> SACKFEEGQDVLARWSDGLFYLGTIKKINILKQSCFIIFEDSSKSWVLWKDIQTGATGSGEMVCTICQEEYSEAPNEMVICDKCGQGYHQLCHTPHIDCSVIDSDEKWLCRQCVFATTTKRGGALKKGPNAKALQVMKQTLPYSV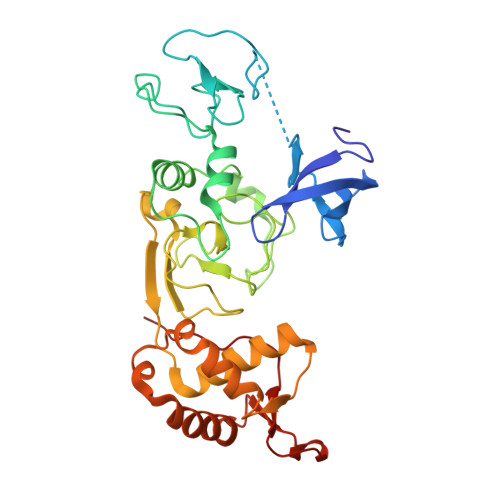ADLEWDAGHKTNVQQCYCYCGGPGDWYLKMLQCCKCKQWFHEACVQCLQKPMLFGDRFYTFICSVCSSGPEYLKRLPLQWVDIAHLCLYNLSVIHKKKYFDSELELMTYINENWDRLHPGELADTPKSERYEHVLEALNDYKTMFMSGKEIKKKKHLFGLRIRVPPVPPNVA>MVNKMDIIPEITRKSITDLINNKERIDGRSLHEFRDISIETGVISKAEGSSRVKLGNTQIIVGVKPQIGEPFPDTPEMGVILTNSELLPMASPTFEPGPPDERSVELSRVVDRCIRESRMIDLEKLCIIEGSKVWMLFLDLHIIDYDGNLFDAAVLATVAALLDTRIPAAEVEDGEVVINREKMQPLPVNRKALMCTFAKIGNEIVLDPSLEEEDILTARISIGVTEEGSICAMQKGGEGPLTRDDVLKAVSIAVEKVPQLIEYLDKSMTP[3x];>MITIITQDQLKTSPSVREDGRAFDELRPLKIEAGILERADGSSYLEFGGNKILVAVYGPREAQIRKLQRPDRAVIRCRYNMAPFSVEERKRPGPDRRSV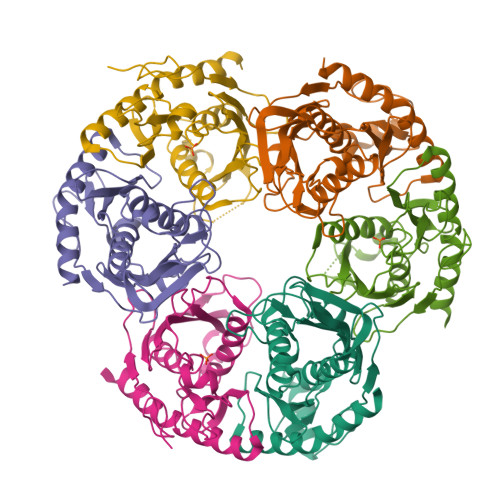EISKITAEALRPALILEKFPRSVIDVFIEVLEAEGGTRCAGITAASVALADAGIPMRDMVVACAAGKVGDQVVLDLSEEEDKEGQADVPVAILPRTREITLLQSDGNLTPEEFERALDLAVEGCLRIHEVQKEALRKRYGE[3x]>ASAWPEEKNYHQPAILNSSALRQIAEGTSISEMWQNDLQPLLIERYPGSPGSYAARQHIMQRIQRLQADWVLEIDTFLSQTPYGYRSFSNIISTLNPTAKRHLVLACHYDSKYFSHWNNRVFVGATDSAVPCAMMLELARALDKKLLSLKTVSDSKPDLSLQLIFFDGEEAFLHWSPQDSLYGSRHLAAKMASTPHPPGARGTSQLHGMDLLVLLDLIGAPNPTFPNFFPNSARWFERLQAIEHELHELGLLKDHSLEGRYFQNYSYGGVIQADHIPFLRRGVPVLHLIPSPFPEVWHTMDDNEENLDESTIDNLNKILQVFVLE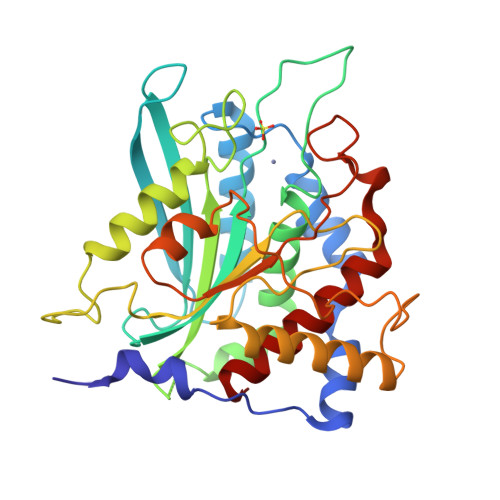YLHL[2x]> GHMFGSLYSDERDKPLLSPTAQKKFEEYQNKLANL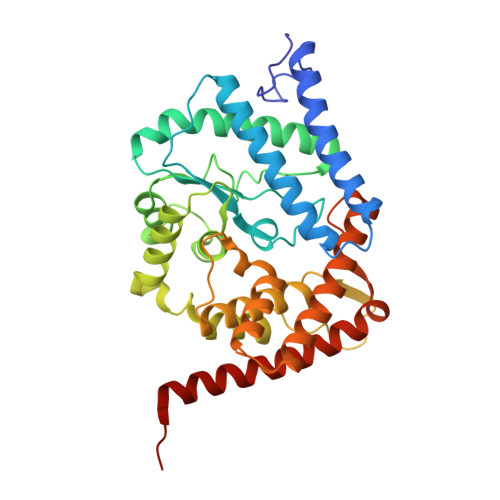SKIIRENEGNEVSPWQEWENGLRQIYKEMIYDAFDALGVEMPKDMEVHFAGSLAKAQATEYSDLDAFVIVKNDEDIKKVKPVFDALNNLCQRIFTASNQIYPDPIGINPSRLIGTPDDLFGMLKDGMVADVEATAMSILTSKPVLPRYECGEELRDKIKQEPSFSNMVSAKKFYNKAIKDFTAPKEGAEVVSVKTHIMRPIDFMLMGLREEFNLYSEDGAHLSAPGTIRLLREKNLLPEEQIARIESVYNQAMSKRFELHAEHKKEHDEMPYSDAKAMLDEVAKIRELGVQRVTRIENLENAKKL> GSFTSSGMEQIQMVKVLEKCQVTPPSDTTDVELSLPVTFFDIPWLHLNKMQSLLFYDFPYPRTHFLDTVIPNLKASLSLTLKHYVPLSGNLLMPIKSGEMPKFQYSRDEGDSITLIVAESDQDFDYLKGHQLVDSNDLHGLFYVMPRVIRTMQDYKVIPLVAVQVTVFPNRGIAVALTAHHSIADAKSFVMFINAWAYINKFGKDADLLSANLLPSFDRSIIKDLYGLEETFWNEMQDVLEMFSRFGSKPP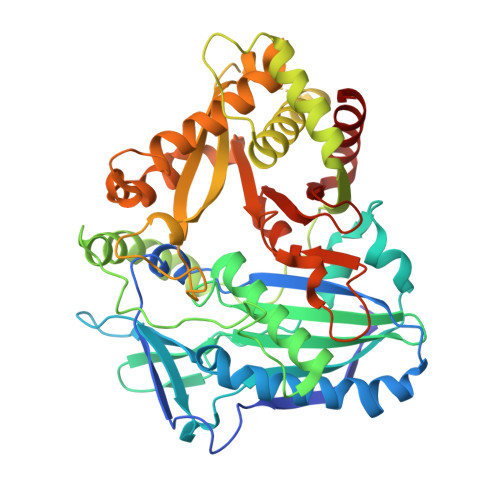RFNKVRATYVLSLAEIQKLKNKVLNLRGSEPTIRVTTFTMTCGYVWTCMVKSKDDVVSEESSNDENELEYFSFTADCRGLLTPPCPPNYFGNCLASCVAKATHKELVGDKGLLVAVAAIGEAIEKRLHNEKGVLADAKTWLSESNGIPSKRFLGITGSPKFDSYGVDFGWGKPAKFDITSVDYAELIYVIQSRDFEKGVEIGVSLPKIHMDAFAKIFEEGFCSLS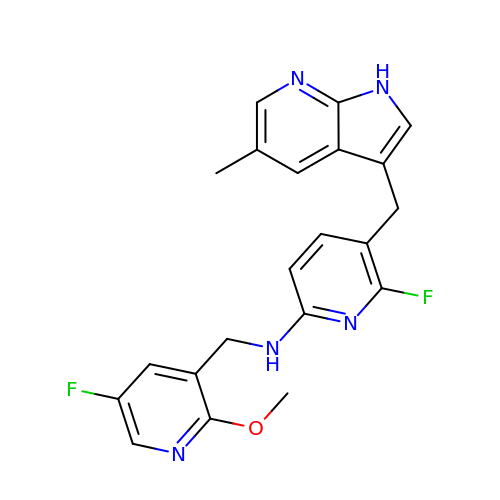6-fluoro-N-[(5-fluoro-2-methoxypyridin-3-yl)methyl]-5-[(5-methyl-1H-pyrrolo[2,3-b]pyridin-3-yl)methyl]pyridin-2-amine | C21 H19 F2 N5 O | NSMOZFXKTHCPTQ-UHFFFAOYSA-N> HHHHHHMRVLGLNGWPRDFHDASAALLVDGRIAAFAEEERFTRKKHGYNTAPVQAAAFCLAQAGLTVDDLDAVAFGWDLPAMYRERLGGWPHSDSEALDILLPRDVFPRRTDPPLHFVQHHLAHAASAYYFSGEDRGAVLIVDGQGEEECVTLAHAEGGKITVLDTVPGAWSLGFFYEHVSEYTGLGGDNPGKLMGLAAHGTTVDETLSAFAFDSDGYRLNLIDPQARDPEDWDEYSVTERAWFAHLERIYRLPPNEFVRRYDPAKGRVVRDTRRDPYEYRDLAAT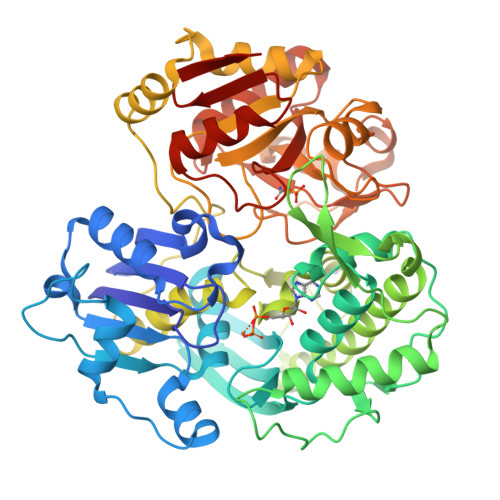AQAALERAVFGLADSVLARTGERTLFVAGGVGLNATMNGKLLTRSTVDKMFVPPVASDIGVSLGAAAAVAVELGDRIAPMGDTAAWGPEFSPDQVRAALDRTGLAYREPANLEREVAALIASGKVVGWAQGRGEVGPRALGQRSLLGSAHSPTMRDHINLRVKDREWWRPFAPSMLRSVSDQVLEVDADFPYIIMTTKVRAAYAERLPSVVHEDWSTRPQTVTEASNPRYHRMLTELGDLVGDPVCLNTSFNDRGEPIVSSPADALLTFSRLPIDALAVGPYLVTKDLRH Previous work has demonstrated that one particular kinase, known as cyclic guanosine-3′,5′-monophosphate (cGMP)-dependent protein kinase, or protein kinase G (PKG), has essential roles in multiple stages of the parasite life cycle. Selective pharmacological inhibition of Plasmodium falciparum PKG (PfPKG) blocks the egress of merozoites and gametes from erythrocytes, as well as inhibits the motility of ookinetes in the mosquito and invasion of hepatocytes by sporozoites. The cellular functions of parasite PKG are regulated by allosteric and cooperative binding of cGMP, similarly to how mammalian PKG is activated. In contrast, PKG enzymes of Plasmodium and other apicomplexan parasites have an extended N-terminal domain that features four CNBs upstream of the KD and are monomeric, resulting in an effective regulatory stoichiometry of 4:1.

To overcome stability issues of PKG in the presence of cGMP, we produced isolated CNBs to capture cGMP-dependent conformational changes in other CNBs. As such, we report the cocrystallized PfCNB-A structure bound to cGMP, which illustrates the reorganization of helix αCA upon cGMP activation. Especially, we denote the probable rearrangement of key interactions upon cGMP activation, particularly the K157–Y694 π-bond interaction (site 2) between the connecting helix αCA and the activation loop in the immediate vicinity of the kinase active site. This clearly suggests a mechanism by which conformational modifications induced by binding of cGMP to one CNB could be relayed to adjacent domains. The conformational alteration of this connecting helix is expected to make a significant contribution to kinase activity, as it makes important interactions with the kinase activation loop (K157–Y694 π-bond stabilization). The torsion of the connecting helix αCA is reminiscent of cAMP-dependent activation by PKA, which uses a similar mechanism to destabilize the extended αCA helix to uncouple CNB-A and -B before dissociation of the complex. In the middle of the β-barrel of CNB-A, -B, and -D is a 24-residue-long phosphate-binding cassette (PBC) featuring the universally conserved glutamate and arginine residues, as well as a short flexible helix, sometimes referred to as the B′-helix. Their interactions with cGMP were determined by isothermal titration calorimetry (ITC), revealing 14, 17, and 0.17 µM binding affinities for the CNB-A, -B, and -D when expressed as standalone recombinant protein samples, respectively.

> GSNDDFTGEDSLMEDHLELREKLSEDIDMIKTSLKNNLVCSTLNDNEILTLSNYMQFFVFKSGNLVIKQGEKGSYFFIINSGKFDVYVNDKKVKTMGKGSSFGEAALIHNTQRSATIIAETDGTLWGVQRSTFRATLKQLSNR> SISQQTVWNQMATVRTPLNFDSSKQSFCQFSVDLLGGGISVDKTGDWITLVQNSPISNLLRVAAWKKGCLMVKVVMSGNAAVKRSDWASLVQVFLTNSNSTEHFDACRWTKSEPHSWELIFPIEVCGPNNGFEMWSSEWANQTSWHLSFLVDNPKQSTTFDVLLGISQNFEIAGNTLMPAFSVP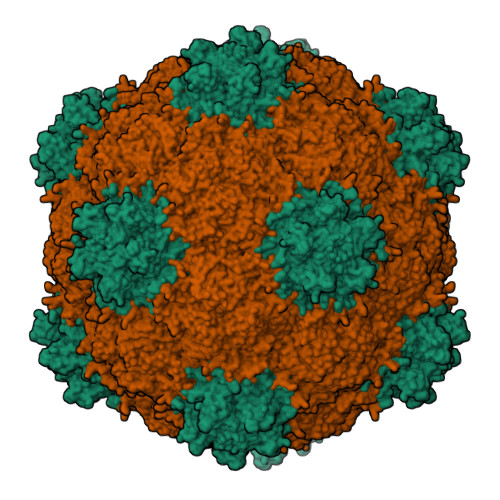Q;> MLDLKISQSKIALPKNTVGGTILRSDLLANFLTEGNFRASVDLQRTHRIKGMIKMVATVGIPENTGIALACAMNSSIRGRASSDIYTICSQDCELWNPACTKAMTMSFNPNPCSDAWSLEFLKRTGFHCDIICVTGWTATPMQDVQVTIDWFISSQECVPRTYCVLNPQNPFVLNRWMGKLTFPQGTSRSVKRMPLSIGGGAGAKSAILMNMPNAVLSMWRYFVGDLVFEVSKMTSPYIKCTVSFFIAFGNLADDTINFEAFPHKLVQFGEIQEKVVLKFSQEEFLTAWSTQVRPATTLLADGCPYLYAMVHDSSVSTIPGDFVIGVKLTIIENMCAYGLNPGISGSRLLG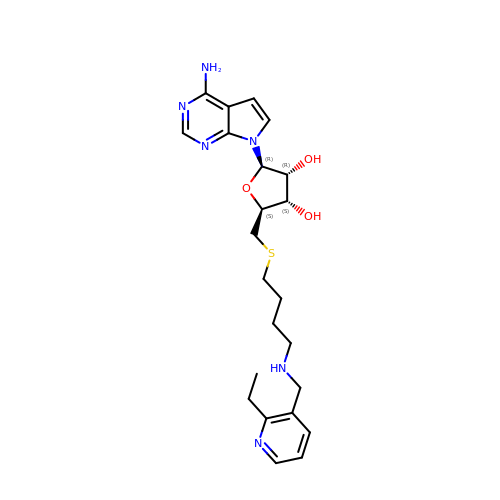7-[5-S-(4-{[(2-ethylpyridin-3-yl)methyl]amino}butyl)-5-thio-beta-D-ribofuranosyl]-7H-pyrrolo[2,3-d]pyrimidin-4-amine | C23 H32 N6 O3 S | SBQBBUZLJIAJBR-GLHSZLCASA-N>MEPKHIINDNVYGTVKVPRPIDKLIDTVEFQRLRHLKQTGLVYLVYPNCEHSRFVHSLGTFSLAYALVDKLRHSQPSLNITESDLICTSVAALLRNVGHGPFSHLFDGEFAKRNGSRFKHEDMSILIIKKIMNKPEIKSEFACILGETDEEYAKSVTLITELISGKPFDFQDMDGFKDLPADVREETVKNEWAIIGCGPEKSFLFDVVSNSYNGHDVDKMDYLLRDSKASGVGITFSESTLERLFNHVRVVIDPNSGLKRIAYSIKCIGDLKAIGDSRQELHSKVYQHKAVRFMETLMVDALINAGDFLKYKGSNGELYSLKNVTEDVDAFLKTTDYVEQEILNSQITDPKMIEAQTALLKIQRREIGCKLGYFEMNPENATQLKGNCNNQTGAAEVVKKVGQKMKEILEQMDDTEEMDGKLKDIQFTVMHSVLGRGLDDKTHPIERQIFYDGKPSEHEGKQVVGFYPSEDYVINNCPRMATKWEIFVMGDRSLRKEPLLADRVKRALQLAGESEKFLTPRKRSPQ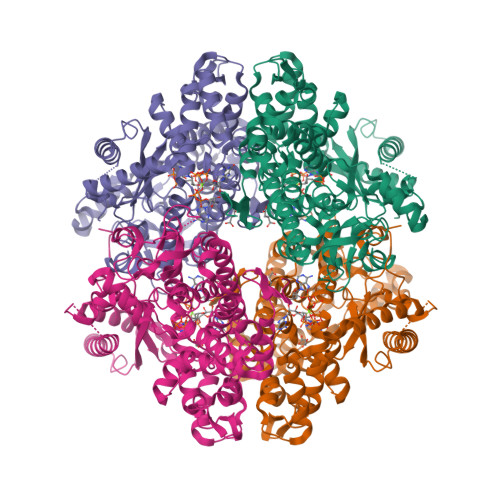[4x]N-[2-(5-methyl-4H-1,2,4-triazol-3-yl)phenyl]-7H-pyrrolo[2,3-d]pyrimidin-4-amine | C15 H13 N7 | 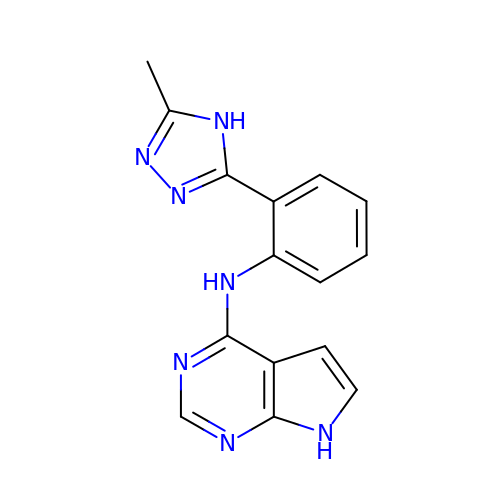OKGCSZUKOGMZAL-UHFFFAOYSA-N>CPRFLKVKNWETEVVLTDTLHLKSTLETGCTEYICMGSIMHPSQHARRPEDVATKDQLFPLAKEFIDQYYSSIKRFGSKAHMERLEEVNKEIDTTSTYQLKDTELIYGAKHAWRNASRCVGRIQWSKLQVFDARDCTTAHGMFNYICNHVKYATNKGNLRSAITIFPQRTDGKHDFRVWNSQLIRYAGYKQPDGSTLGDPANVQFTEICIQQGWKPPRGRFDVLPLLLQANGNDPELFQIPPELVLEVPIRHPKFEWFKDLGLKWYGLPAVSNMLLEIGGLEFSACPFSGWYMGTEIGVR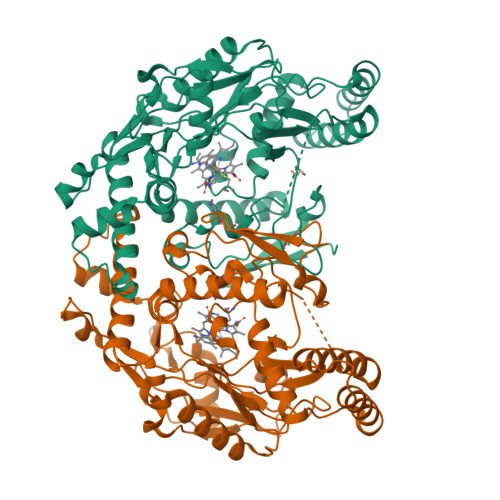DYCDNSRYNILEEVAKKMNLDMRKTSSLWKDQALVEINIAVLYSFQSDKVTIVDHHSATESFIKHMENEYRCRGGCPADWVWIVPPMSGSITPVFHQEMLNYRLTPSFEYQPDPWNTHVWK[2x]>[2x]TNATGERNLALIQEVLEVFPETARKE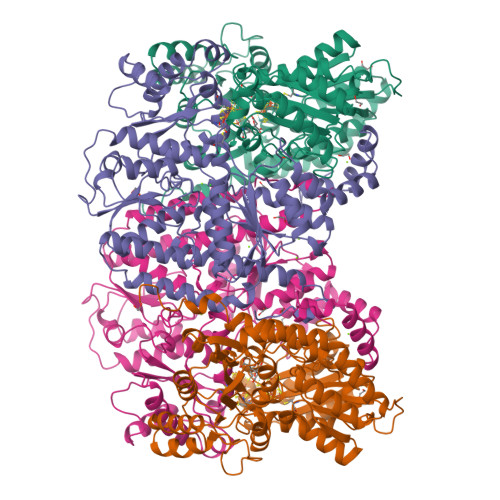RRKHMMVSDPKMKSVGKCIISNRKSQPGVMTVRGCAYAGSKGVVFGPIKDMAHISHGPVGCGQYSRAGRRNYYTGVSGVDSFGTLNFTSDFQERDIVFGGDKKLSKLIEEMELLFPLTKGITIQSECPVGLIGDDISAVANASSKALDKPVIPVRCEGFRGVSQSLGHHIANDVVRDWILNNREGQPFETTPYDVAIIGDYNIGGDAWASRILLEEMGLRVVAQWSGDGTLVEMENTPFVKLNLVHCYRSMNYIARHMEEKHQIPWMEYNFFGPTKIAESLRKIADQFDDTIRANAEAVIARYEGQMAAIIAKYRPRLEGRKVLLYMGGLRPRHVIGAYEDLGMEIIAAGYEFAHNDDYDRTLPDLKEGTLLFDDASSYELEAFVKALKPDLIGSGIKEKYIFQKMGVPFRQMHSWDYSGPYHGYDGFAIFARDMDMTLNNPAWNELTAPWL;>[2x]SQTIDKINSCYPLFEQDEYQELFRNKRQLEEAHDAQRVQEVFAWTTTAEYEALNFRREALTVDPAKACQPLGAVLCSLGFANTLPYVHGSQGCVAYFRTYFNRHFKEPIACVSDSMTEDAAVFGGNNNMNLGLQNASALYKPEIIAVSTTCMAEVIGDDLQAFIANAKKDGFVDSSIAVPHAHTPSFIGSHVTGWDNMFEGFAKTFTADYQGQPGKLPKLNLVTGFETYLGNFRVLKRMMEQMAVPCSLLSDPSEVLDTPADGHYRMYSGGTTQQEMKEAPDAIDTLLLQPWQLLKSKKVVQEMWNQPATEVAIPLGLAATDELLMTVSQLSGKPIADALTLERGRLVDMMLDSHTWLHGKKFGLYGDPDFVMGLTRFLLELGCEPTVILSHNANKRWQKAMNKMLDASPYGRDSEVFINCDLWHFRSLMFTRQPDFMIGNSYGKFIQRDTLAKGKAFEVPLIRLGFPLFDRHHLHRQTTWGYEGAMNIVTTLVNAVLEKLDSDTSQLGKTDYSFDLVR> HMGEQFCVRIEKNPGLGFSISGGISGQGNPFKPSDKGIFVTRVQPDGPASNLLQPGDKILQANGHSFVHM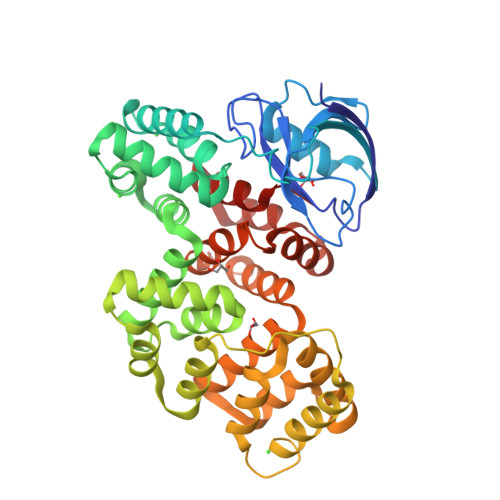EHEKAVLLLKSFQNTVDLVIQRELTGSAYGSVKAYTNFDAERDALNIETAIKTKGVDEVTIVNILTNRSNEQRQDIAFAYQRRTKKELASALKSALSGHLETVILGLLKTPAQYDASELKASMKGLGTDEDSLIEIICSRTNQELQEINRVYKEMYKTDLEKDIISDTSGDFRKLMVALAKGRRAEDGSVIDYELIDQDARDLYDAGVKRKGTDVPKWISIMTERSVPHLQKVFDRYKSYSPYDMLESIRKEVKGDLENAFLNLVQCIQNKPLYFADRLYDSMKGKGTRDKVLIRIMVSRSEVDMLKIRSEFKRKYGKSLYYYIQQDTKGDYQKALLYLCGGDD>[2x]GIDPFTSTQTAEDKEEPLHSIISSTESVQGSTSKHEFQAETKKLLDIVARSLYSEKEVFIRELISNASDALEKLRHKL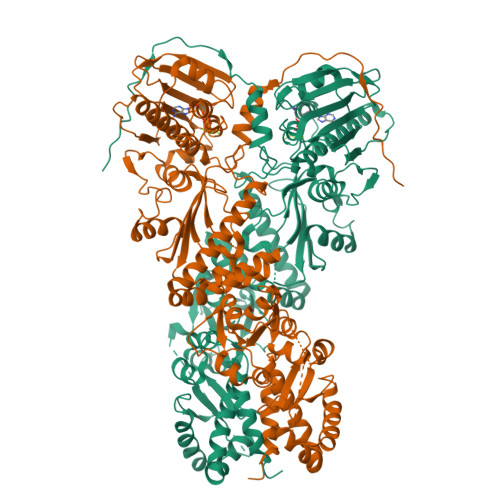VSDGQALPEMEIHLQTNAEKGTITIQDTGIGMTQEELVSNLGTIARSGSKAFLDALQNQAEASSKIIGQFGVGFYSAFMVADRVEVYSRSAAPGSLGYQWLSDGSGVFEIAEASGVRTGTKIIIHLKSDCKEFSSEARVRDVVTKYSNFVSFPLYLNGRRMNTLQAIWMMDPKDVGEWQHEEFYRYVAQAHDKPRYTLHYKTDAPLNIRSIFYVPDMKPSMFDVSRELGSSVALYSRKVLIQTKATDILPKWLRFIRGVVDSEDIPLNLSRELLQESALIRKLRDVLQQRLIKFFIDQSKKDAEKYAKFFEDYGLFMREGIVTATEQEVKEDIAKLLRYESSALPSGQLTSLSEYASRMRAGTRNIYYLCAPNRHLAEHSPYYEAMKKKDTEVLFCFEQFDELTLLHLREFDKKKLISVETDIVVDHYKEEKFEDRSPAAECLSEKETEELMAWMRNVLGSRVTNVKVTLRLDTHPAMVTVLEMGAARHFLRMQQLAKTQEERAQLLQPTLEINPRHALIKKLNQLRASEPGLAQLLVDQIYENAMIAAGLVDDPRAMVGRLNELLVKALERHGGSGSGSSAMVDTLSGLSSEQGQSGDMTIEEDSATHIKFSKRDEDGKELAGATMELRDSSGKTISTWISDGQVKDFYLYPGKYTFVETAAPDGYEVATAITFTVNEQGQVTVNGKATKGDAHI>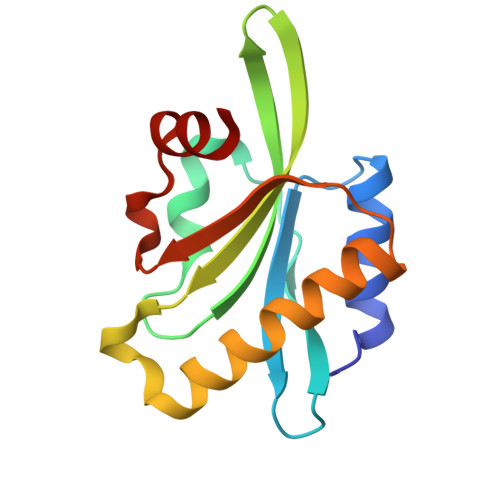 SMPLQPEAQRALQQLKQKMVNYIQMKLDLERETIELVHTEPTDVAQLPSRVPRDAARYHFFLYKHTHEGDPLESVVFIYSMPGYKCSIKERMLYSSCKSRLLDSVEQDFHLEIAKKIEIGDGAELTAEFLDDEVH Processing of coproporphyrinogen to heme b takes three steps in both pathways, but in the CPD pathway decarboxylation of the propionate groups to the vinyl groups is the ultimate step and is catalyzed by the enzyme coproheme decarboxylase (ChdC), which does not have an analogous enzyme in the PPD pathway. CpfCs are members of class II chelatases, which are ATP-independent monomeric or dimeric enzymes. In order to understand the enzymatic mechanism of CpfCs, we combined biochemical and crystal structure analyses of CpfC from Listeria monocytogenes (LmCpfC) in its apo-form and the product-bound state with iron coproporphyrin III (coproheme). The polypeptide is folded into a monomeric protein with two ferredoxin-like domains each with a four-stranded parallel β-sheet flanked by α-helices.

Diffraction data for apo- and coproheme-LmCpfCs were collected to 1.64 Å resolution. Structures were solved with molecular replacement using BsCpfC, the structurally best studied representative from Firmicutes ferrochelatases, as a search model, and refined to Rfree values of 0.2013 (apo-LmCpfC) and 0.2014 (coproheme-LmCpfC); for complete data collection and refinement statistics, please see Table 1. In the apo-structure, the substrate/product binding site is occupied by solvent molecules (phosphates and glycerols). Interestingly, the orientation of Glu263 is notably different compared to the product bound, pointing away from the His182. In the apo-protein, the active site (i.e., coproporphyrin III binding site) is filled with solvent molecules that are released upon binding of the macrocycle as seen in the crystal structures of apo-LmCpfC and coproheme-LmCpfC. In the apo-structure, the side chain of Ser53 is solvent exposed, while in the product-bound form, it points to the inner core of the protein, due to the interaction with p4. Similarly, Arg45 (H-bond to p6) adopts a notably different conformation in the apo-structure compared to the coproheme-bound structure, even though it is hydrogen bonded to Asp41 in both cases. The H-bonding pattern changes from one H-bond in the apo-form to a bidentate binding to the guanidinium group in the holo form. CAVER calculations of the putative substrate channels in apo- and coproheme-LmCpfC show that the throughput (throughput values range from 0 to 1; the higher the value, the greater the importance of the tunnel) for the two calculated main channels in the apo-structure is higher than for the coproheme structure (apo: 0.867 and 0.799; coproheme: 0.832 and 0.757). Additionally, the bottleneck radii for channels in apo-LmCpfC are larger (2.6 and 2.3 Å) than in coproheme-LmCpfC (2.2 and 2.0 Å).

> MTKKVGLLVMAYGTPYKDEDIERYYTDIRHGHKPSEEMIADLRGRYHAIGGLSPLAKITEAQAYGLEKALNDSQDEVEFKAYIGLKHIEPFIEDAVEAMHKDGIEEAISIVLAPHYSSFSVEAYNKRAKEAADKLGGPRINAINDWYKQPKFIQMWADRINETAKQIPADELLDTVLIVSAHSLPEKIKQHNDPYPNQLQETADFIFEKVVVPHYALGWQSEGKTGEPWLGPDVQDLTRELYGREKYKHFIYTPVGFVAEHLEVLYDNDYECKVVTDEVGAAYHRPPMPNSDPEFLEVLRTVVWEKYSNLEH>MKTEQQIADIVNRTITPLMQEQAIPGMAVAVIYQGKPYYFTWGKADIANNHPVTQQTLFELGSVSKTFNGVLGGDAIARGEIKLSDPVTKYWPELTGKQWQGIRLLHLATYTEGGLPLKIPDDVRDKAALLHFYQNWQPQWTPGAKRLYANSSIGLFGALAVKPSGMSYEEAMTRRVLQPLKLAHTWITVPQNEQKDYAWGYREGKPVHSSPGQLDAEAYGVKSSVIDMARWVQANMDASHVQEKTLQQGIALAQSRYWRIGDMYQGLGWEMLNWPLKADSIINGSDSKVALAALPAVEVNPPAPAV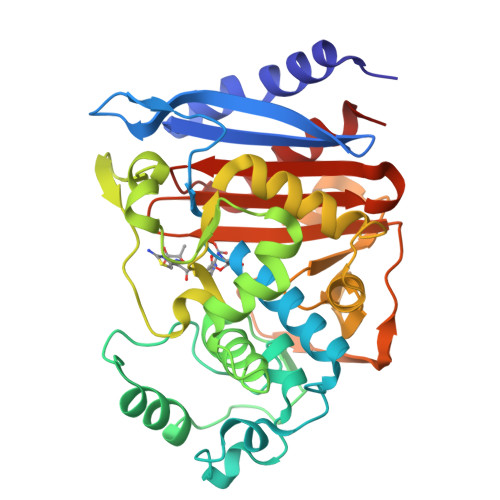KASWVHKTGSTGGFGSYVAFVPEKNLGIVMLANKSYPYPVRVEAAWRILEKLQ[2x]>[2x]GSHMSRILAVHASPRGERSQSRRLA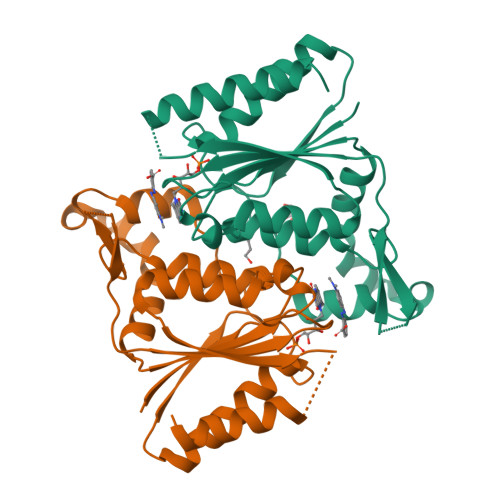EVFLAAYREAHPQARVARREVGRVPLPAVTEAFVAAAFHPQPEQRSLAMQADLALSDQLVGELFDSDLLVISTPMYNFSVPSGLKAWIDQIVRLGVTFDFVLDNGVAQYRPLLRGKRALIVTSRGGHGFGPGGENQAMNHADPWLRTALGFIGIDEVTVVAAEGEESGGRSFEDSCDEAEQRLLALARSA> TINVTGDGNVFKPSAETSSTAVPSLSLSPGMLNPGGVPWIAIGDETSVTSPGALRRMTSKDIDEPLVVVTEHAIANFTKAEMALEFNREFLDKLRVLSVSPKYSDLLTYVDCYVGVSARQALNNFQKQVPVITPTRQTMYVDSIQAALKALEKWEIDLRVAQTLLPTNVPIGEVSCPMQSVVKLLDDQLPDDSLIRRYPKEAAVALAKRNGGIQWMDVSEGTVMNEAVNAVAASALAPSASAPPLEEKSKLTEQAMDLVTAAEPEIIASLVPVPAPVFAIPPKPADYNVRTLKIDEATWLRMIPKTMGTLFQIQVTDNTGTNWHFNLRGGTRVVNLDQIAPMRFVLDLGGKSYKETSWDPNGKKVGFIVFQSKIPFELWTAASQIGQATVVNYVQLYAEDSSFTAQSIIATTSLAYNYEPEQLNKTDPEMNYYLLATFIDSAAITPTNMTQPDVWDA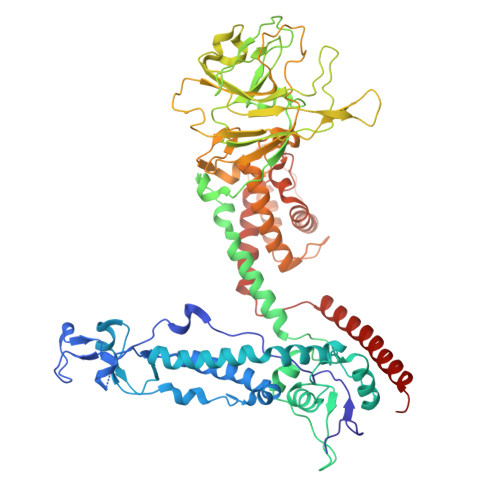LLTMSPLSAGEVTVKGAVVSEVVPAELIGSYTPESLNASLPNDAARCMIDRASKIAEAIKIDDDAGPDEYSPNSVPIQGQLAISQLETGYGVRIFNPKGILSKIASRAMQAFIGDPSTIITQAAPVLSDKNNWIALAQGVKTSLRTKSLSAGVKTAVSKLSSSESIQNWTQGFLDKVSTHFPAP>MGAAILPDLGTEILIPVCAVIGIAFALFQWLLVSKVKLSAVRDASPNAAAKNGYNDYLIEEEEGINDHNVVVKCAEIQNAISEGATSFLFTEYKYVGIFMVAFAILIFLFLGSVEGFSTSPQACS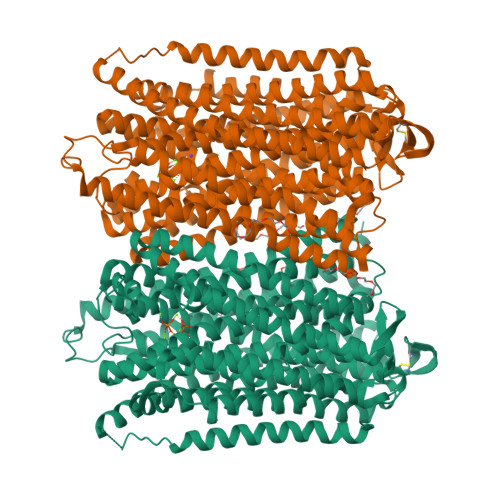YDKTKTCKPALATAIFSTVSFLLGGVTSLVSGFLGMKIATYANARTTLEARKGVGKAFITAFRSGAVMGFLLAANGLLVLYIAINLFKIYYGDDWGGLFEAITGYGLGGSSMALFGRVGGGIYTKAADVGADLVGKVERNIPEDDPRNPAVIADNVGDNVGDIAGMGSDLFGSYAESSCAALVVASISSFGLNHELTAMLYPLIVSSVGILVCLLTTLFATDFFEIKAVKEIEPALKKQLVISTVLMTIGVAVVSFVALPTSFTIFNFGVQKDVKSWQLFLCVAVGLWAGLIIGFVTEYYTSNAYSPVQDVADSCRTGAATNVIFGLALGYKSVIIPIFAIAISIFVSFTFAAMYGIAVAALGMLSTIATGLAIDAYGPISDNAGGIAEMAGMSHRIRERTDALDAAGNTTAAIGKGFAIGSAALVSLAKFGAFVSRASITTVDVLTPKVFIGLIVGAMLPYWFSAMTMKSVGSAALKMVEEVRRQFNTIPGLMEGTAKPDYATCVKISTDASIKEMIPPGALVMLTPLVVGILFGVETLSGVLAGSLVSGVQIAISASNTGGAWDNAKKYIEAGASEHARSLGPKGSDCHKAAVIGDTIGDPLKDTSGPSLNILIKLMAVESLVFAPFFATHGGLLFKIF[2x]Here we report three-dimensional structures of three large ornate bacterial RNAs using cryo-electron microscopy (cryo-EM). GOLLD (Giant, Ornate, Lake- and Lactobacillales-Derived), ROOL (Rumen-Originating, Ornate, Large) and OLE (Ornate Large Extremophilic) RNAs form homo-oligomeric complexes whose stoichiometries are retained at lower concentrations than measured in cells. Unexpectedly, the three structures are stabilized not by proteins but by other copies of the same RNA molecule in ornate quaternary assemblies with many intermolecular bridges, a phenomenon that has not previously been observed for natural RNA molecules. Extensive intramolecular and intermolecular A-minor interactions, kissing loops, an unusual A–A helix and other interactions stabilize the three complexes.

OLE is a class of large RNAs with an ornate secondary structure that is conserved throughout evolution. Furthermore, a 2.9 Å resolution 3D map of a dimeric OLE RNA could be reconstructed with two-fold imposed symmetry. Our OLE dimer map shows that it is organized as a series of parallel A-form helices, resembling a bundle of pipes. An unusual but highly conserved symmetric interaction comprised of four A–A base pairs between two chains (L4), intermolecular base pairing and stacking interactions connecting L5, L6 and L7, and a kissing loop (L9.3) ‘weld’ the pipes together in the middle of the complex. Beyond the 5′ region, other conserved parts of OLE were not resolved in the structure, suggesting flexibility. Surprisingly, regions of OLE that were previously thought to adopt alternative structures upon protein binding are clearly resolved and solvent-accessible, suggesting that proteins may bind the OLE dimer in the pre-formed RNA conformation that we observed here. Our cryo-EM data show that these proteins are not required for the folding of the 5′ domain of OLE, and the RNA structure itself may have a crucial role in organizing these proteins. A163 is flipped out of the helix and docks into a pocket created by P5, P6, P7 and dimer interface. This OLE dimer pocket is reminiscent of the pocket RpsU occupies in the ribosome, supporting the previous hypothesis that OLE could sequester RpsU15. OLE forms a dimer shaped like a bundle of pipes and exposes structured binding pockets for protein partners such as the membrane-associated OLE-associated protein A (OapA).

>[2x]GGUGCAGUAUUCUAGUCAGGGAAAUGCUUUUUGAAGGCGGGGCUAAAAAUCCGCUAAAGGGCACAUCGAUGAAGUUCCUGGUGCUGGCCUUAGAAUGCCCAGUCUUGGGCUUGUGCUGGGAGUUAAAAAAGCUGGGGCACUCGCAAUGGCAUGCGACAAAUGACCCUACUUUUGUGGAGGCCAAUUAUUGUAUAUUGAGAGAGAUAUUCAAUAUACGAAAUUGGGGUAAACCUGCAAUGUGGUGUAAAAGCUAUGUGCAGUGUAGCCUGCCUUGAGUGGUAUGGGGAGAGGAGAUAAACAAGUCAAAAAUUUUAGGCCUAAGUUUUUGUACUAUUGAACUCUGAAACCUAUGUUGCAAAAGAGGCUAAGAAAGCAUCUAACUGUUGAGGAAAACUCCUAGACUGUUUUGGUAAAAUGAGGAUUGCAGUGCGGACUUAGUGGCAAUUCAGUCCUGAAAGUGGCAACACUUCAGCUCGGAUAUUAAAGGGAAACCGCUAUAUGGCGACGUAUAGUUAUUCGUGGGGAAAGCCUACUGAACCUAUGCCGUAAGAUUUACUUAUUUUGUUACCACAUUGCC[(2~{R},3~{S},4~{R},5~{R})-5-(6-aminopurin-9-yl)-2-[[[(2~{R},3~{S},4~{R},5~{R})-5-(2-azanyl-6-oxidanylidene-1~{H}-purin-9-yl)-2-(hydroxymethyl)-4-oxidanyl-oxolan-3-yl]oxy-sulfanyl-phosphoryl]oxymethyl]-4-oxidanyl-oxolan-3-yl]oxy-sulfanyl-phosphinic acid | C20 H26 N10 O12 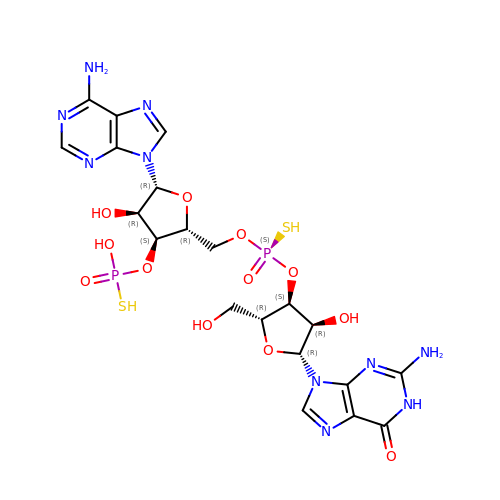P2 S2 | MLCQGAYMLYXJTJ-WEKBUWATSA-N> MVNYTFIDKRVIKRTTMIEGDVETVSPLKIGGGKDNFDPSSLAKDSILKDVEGRPIIPGSSWKGIFRSTGERILRLRNIEVCSGIGKDYCLNNNRKERDFNSALKENVDQALEIFWDYTCLNCKVFGTMSVIGAVRFLDSLPISYSLNTRSMIAISRTEGAVARRALVTVEYVDV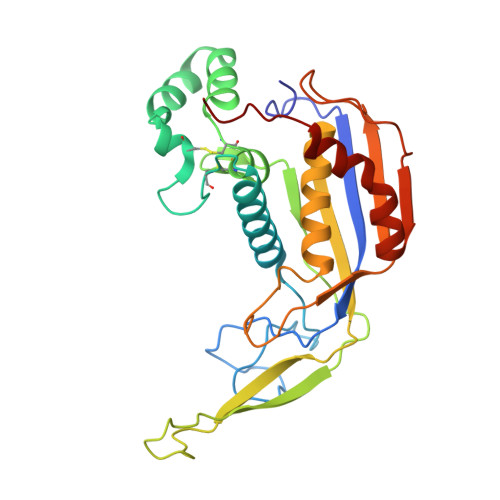GSKFSFKMMGYNLPNYAIGYLITIMKNIHDGFTQVGGHKSRGFGFVKFGKVKFTDLGEKRIGDEDIQVKDVGDLVEGNGDEFFGRMKPFMEAFNNAKIPYPKK AMPylation (adenylylation) is an evolutionarily conserved PTM characterized by the covalent addition of adenosine monophosphate (AMP) to the hydroxyl side chains of amino acids in protein substrates. We developed a strategy to enrich for AMPylated proteins using the histidine triad nucleotide-binding protein, hinT. Although its physiological substrates are still unknown, in vitro characterization of hinT revealed high-affinity purine nucleotide binding and phosphoramidase activity. To investigate the structural mechanisms of AMPylated protein binding to hinTHN, we used AMPylated GlnA (GlnA-AMP) as a model substrate.

GlnA forms a dodecamer composed of two hexameric rings that is ideal for cryo-electron microscopy (cryo-EM) analysis. The cryo-EM structure of hinT H101N bound to GlnA revealed up to six hinT dimers bound to the external surface of GlnA dodecamer. A Cryo-EM density map representation of the GlnA-hinT H101N complex. The dodecamer GlnA is in blue and the dimeric hinT H101N is in pink.

>[12x]SEFELMSAEHVLTMLNEHEVKFVDLRFTDTKGKEQHVTIPAHQVNAEFFEEGKMFDGSSIGGWKGINESDMVLMPDASTAVIDPFFADSTLIIRCDILEPGTLQGYDRDPRSIAKRAEDYLRSTGIADTVLFGPEPEFFLFDDIRFGSSISGSHVAIDDIEGAWNSSTQYEGGNKGHRPAVKGGYFPVPPVDSAQDIRSEMCLVMEQMGLVVEAHHHEVATAGQNEVATRFNTMTKKADEIQIYKYVVHNVAHRFGKTATFMPKPMFGDNGSGMHCHMSLSKNGVNLFAGDKYAGLSEQALYYIGGVIKHAKAINALANPTTNSYKRLVPGYEAPVMLAYSARNRSASIRIPVVSSPKARRIEVRFPDPAANPYLCFAALLMAGLDGIKNKIHPGEAMDKNLYDLPPEEAKEIPQVAGSLEEALNELDLDREFLKAGGVFTDEAIDAYIALRREEDDRVRMTPHPVEFELYYSV> MHPGFFTSIGQMTDLIHTEKDLVTSLKDYIKAEEDKLEQIKKWAEKLDRLTSTATKDPEGFVGHPVNAFKLMKRLNTEWSELENLVLKDMSDGFISNLTIQ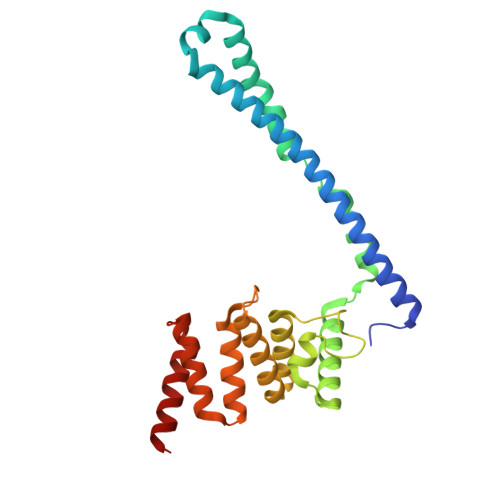RQYFPNDEDQVGAAKALLRLQDTYNLDTDTISKGNLPGVKHKSFLTAEDCFELGKVAYTEADYYHTELWMEQALRQLDEGEISTIDKVSVLDYLSYAVYQQGDLDKALLLTKKLLELDPEHQRANGNLKYFEYIMAKE>HHHHHHMQFVNKQFNYKDPVNGVDIAYIKIPNAGQMQPVKAFKIHNKIWVIPERDTFTNPEEGDLNPPPEAKQVPVSYYDSTYLSTDNEKDNYLKGVTKLFERIYSTDLGRMLLTSIVRGIPFWGGSTIDTELKVIDTNCINVIQPDGSYRSEELNLVIIGPSADIIQFECKSFGHEVLNLTRNGYGSTQYIRFSPDFTFGFEESLEVDTNPLLGAGKFATDPAVTLAHELIHAGHRLYGIAINPNRVFKVNTNAYYEMSGLEVSFEELRTFGGHDAKFIDSLQENEFRLYYYNKFKDIASTLNKAKSIVGTTASLQYMKNVFKEKYLLSEDTSGKFSVDKLKFDKLYKMLTEIYTEDNFVKFFKVLNRKTYLNFDKAVFKINIVPKVNYTIYDGFNLRNTNLAANFNGQNTEINNMNFTKLKNFT[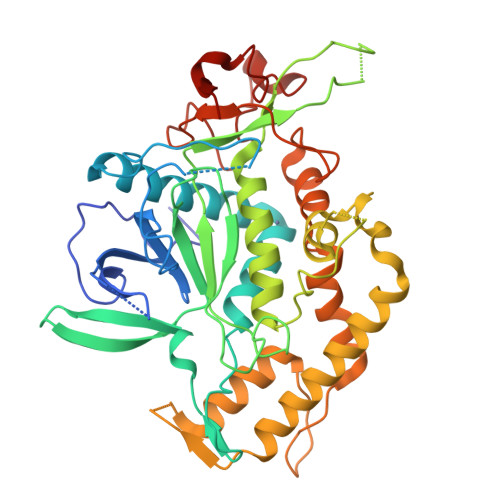2x]>MTFISRFAPDQPRKGADILVEALERQGVETVFAYPGGASMEIHQALTRSSSIRNVLPRHEQGGVFAAEGYARSSGKPGICIATSGPGATNLVSGLADALLDSVPLVAITGQVPRRMIGTDAFQETPIVEVTRSITKHNYLVMDVEDIPRIIEEAFFLATSGRPGPVLVDVPKDIQQQLAIPNWEQAMRLPGYMSRMPKPPEDSHLEQIVRLISESKKPVLYVGGGCLNSSDELGRFVELTGIPVASTLMGLGSYPCDDELSLHMLGMHGTVYANYAVEHSDLLLAFGVRFDDRVTGKLEAFASRAKIVHIDIDSAEIGKNKTPHVSVCGDVKLALQGMNKVLENRAEELKLDFGVWRNELNVQKQKFPLSFKTFGEAIPPQYAIKVLDELTDGKAIISTGVGQHQMWAAQFYNYKKPRQWLSSGGLGAMGFGLPAAIGASVANPDAIVVDIDGDGSFIMNVQELATIRVENLPVKVLLLNNQHLGMVMQWEDRFYKANRAHTFLGDPAQEDEIFPNMLLFAAACGIPAARVTKKADLREAIQTMLDTPGPYLLDVICPHQEHVLPMIPSGGTFNDVITEGDGRIKY[8x];>MAAISVSSSPSIRCLRSACSDSSPALVSSTRVSFPAKISYLSGISSHRGDEMGKRMEGFVRSVDGKISDASFSEASSATPKSKVRKHTISVFVGDESGMINRIAGVFARRGYNIESLAVGLNRDKALFTIVVCGTERVLQQVIEQLQKLVNVLKVEDISSEPQVERELMLVKVNAHPESRAEIMWLVDTFRARVVDIAEHALTIEVTGDPGKMIAVERNLKKFQIREIVRTGKIALRREKMGATAPFWRFSAASYPDLKEQAPVSVLRSSKKGAIVPQKETSAGGDVYPVEPFFDPKVHRILDAHWGLLTDEDTSGLRSHTLSLLVNDIPGVLNIVTGVFARRGYNIQSLAVGHAETKGISRITTVIPATDESVSKLVQQ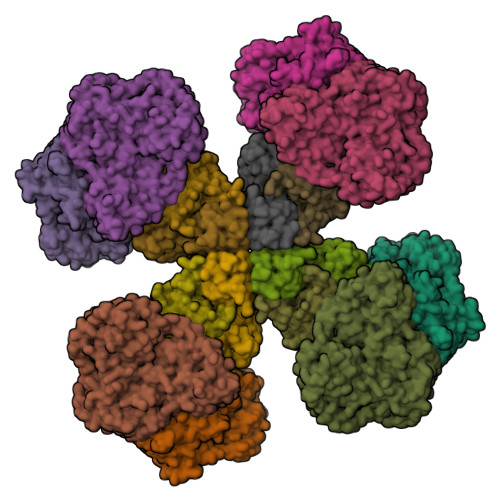LYKLVDVHEVHDLTHLPFSERELMLIKIAVNAAARRDVLDIASIFRAKAVDVSDHTITLQLTGDLDKMVALQRLLEPYGICEVARTGRVALARESGVDSKYLRGYSFPLTG[8x]> GVPTYLLPGSGQFLTTDDHSSAPVLPCFNPTPEMHIPGQVRNMLEVVQVESMMEINNTESAVGMERLKVDISALTDVDQLLFNIPLDIQLDGPLRNTLVGNISRYYTHWSGSLEMTFMFCGSFMATGKLILCYTPPGGSCPTTRETAMLGTHVVWDFGLQSSVTLIIPWISGSHYRMFNNDAKSTNANVGYVT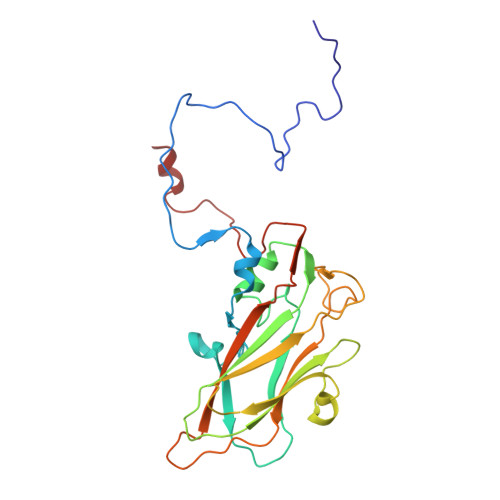CFMQTNLIVPSESSDTCSLIGFIAAKDDFSLRLMRDSPDIGQLDHLHAAEAAYQ>MKTIKDRIAKWSAIGLLSAVAATAFYAPSASAHGEKSQAAFMRMRTIHWYDLSWSKEKVKINETVEIKGKFHVFEGWPETVDEPDVAFLNVGMPGPVFIRKESYIGGQLVPRSVRLEIGKTYDFRVVLKARRPGDWHVHTMMNVQGGGPIIGPGKWITVEGSMSEFRNPVTTLTGQTVDLENYNEGNTYFWHAFWFAIGVAWIGYWSRRPIFIPRLLMVDAGRADELVSATDRKVAMGFLAATILIVVMAMSSANSKYPITIPLQAGTMRGMKPLELPAPTVSVKVEDATYRVPGRAMRMKLTITNHGNSPIRLGEFYTASVRFLDSDVYKDTTGYPEDLLAEDGLSVSDNSPLAPGETRTVDVTASDAAWEVYRLSDIIYDPDSRFAGLLFFFDATGNRQVVQIDAPLIPSFM[3x];>MSAAQSAVRSHAEAVQVSRTIDWMALFVVFFVIVGSYHIHAMLTMGDWDFWSDWKDRRLWVTVTPIVLVTFPAAVQSYLWERYRLPWGATVCVLGLLLGEWINRYFNFWGWTYFPINFVFPASLVPGAIILDTVLMLSGSYLFTAIVGAMGWGLIFYPGNWPIIAPLHVPVEYNGMLMSIADIQGYNYVRTGTPEYIRMVEKGTLRTFGKDVAPVSAFFSAFMSILIYFMWHFIGRWFSNERFLQST[3x];>[3x]MHETKQGGEKRFTGAICRCSHRYNSMEVKMAATTIGGAAAAEAPLLDKKWLTFALAIYTVFYLWVRWYEGVYGWSAGLDSFAPEFETYWMNFLYTEIVLEIVTASILWGYLWKTRDRNLAALTPREELRRNFTHLVWLVAYAWAIYWGASYFTEQDGTWHQTIVRDTDFTPSHIIEFYLSYPIYIITGFAAFIYAKTRLPFFAKGISLPYLVLVVGPFMILPNVGLNEWGHTFWFMEELFVAPLHYGFVIFGWLALAVMGTLTQTFYSFAQGGLGQSLCEAVDEGLIAK

Methane-oxidizing bacteria play a central role in greenhouse gas mitigation and have potential applications in biomanufacturing. Their primary metabolic enzyme, particulate methane monooxygenase (pMMO), is housed in copper-induced intracytoplasmic membranes (ICMs), of which the function and biogenesis are not known. Activation of the 105 kcal/mol methane C-H bond and oxidation to methanol is accomplished by methane monooxygenase (MMO) enzymes at ambient temperature and pressure. Structural studies of pMMO have focused on a single biological assembly: a 300 kDa trimer comprising three copies each of subunits PmoA, PmoB, and PmoC. The pMMO trimer, resolved by cryoET and subtomogram averaging to 4.8 Å in the ICM, forms higher-order hexagonal arrays in intact cells.

To investigate pMMO in its native environment without the use of detergent, we conducted cryoET STA of pMMO embedded within isolated M. capsulatus (Bath) membranes. The cryoET STA structure of the pMMO trimer embedded in the ICM was determined to 4.8 Å resolution, and is consistent with the structure in native nanodiscs. The trimer architecture and folds of PmoA, PmoB, and PmoC resemble the previous crystal and cryoEM structures. Densities corresponding to regions of PmoA and PmoC not resolved crystallographically are apparent in the map, including part of PmoA (dashed pink ovals) and segments of two highly conserved PmoC helices facing the interior of the trimer (M219 to L254) (dashed cyan oval). These regions were fully modelled in the recent cryoEM structure of pMMO in native nanodiscs, which fits the cryoET STA map well. Several densities not accounted for by the pMMO model are also present and potentially correspond to lipids. Although the side chains are not resolved at 4.8 Å resolution, density corresponding to the backbone of the helices is present in our cryoET STA map from native ICMs. CryoET of these membrane vesicles reveals that the ring-like particles are organized into an ordered hexagonal array. Analysis of the four distinct trimer interfaces contained within the system over a 100-ns simulation showed several interactions between the PmoB soluble domains of adjacent pMMO trimers, including a strong salt bridge interaction between K60 and E338 as well as more transient interactions involving residues K58/E160 and R167/D339. There is a moderate degree of conservation for K60 and E338, while other pairs are less conserved. No direct protein interactions were observed within the transmembrane domains of PmoA, PmoB, or PmoC, suggesting that the inter-trimer contacts responsible for array formation are primarily mediated by the PmoB soluble domains.PROPANE 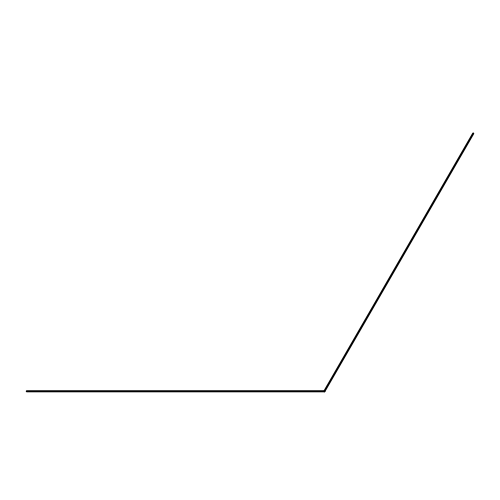| C3 H8 | ATUOYWHBWRKTHZ-UHFFFAOYSA-N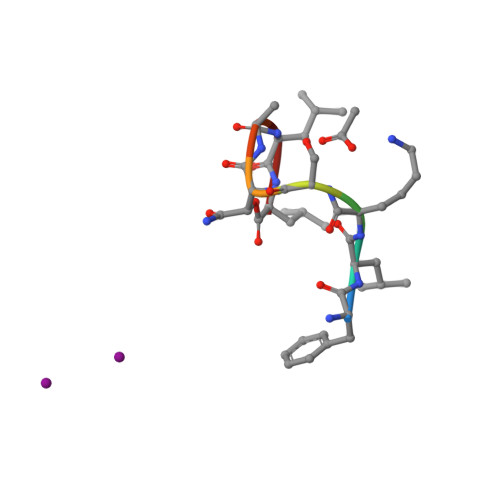>[2x]FLKSXALL>[2x]MAATVWQPLNPGAGGQVQDVVADPNQANVVYMASDMEGVYKSTNNGESWQITGNLVNNRVFAVA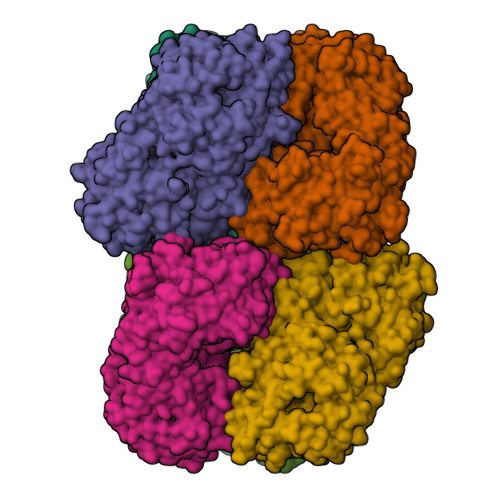VTPGNSNKIFVGTLYGLHISTNGSNSYALVPETENKSIASIAFKPGNANHIIAAPGWRDDDDFIGKFGETAAGPGQVFVSQNGGSSWQTVTFDSNSSTDRNVYSVVFDQSNANTVYLGSNKGVYKSTNGGLNWQRIAGPDDAVRPWNKGIALSPNGQVLYATYAEAKPDLRYNTNFLVYATRTSNINWQQVTGGLEGNRRYWYPEVDPRSTGNSHKVLLGAVKDRFGLYEGTFNWDNNGNLTNFYWEKIWDSYDGSWDIGWDYATPPNARFAHYTPVTGGWARGVWSTTNQTMYYASHNSGNNSYSWQNKYSTPTSQTVNWYGTEWPTYKGKGTESTYTYDVAVHENYVIQGQADNGLMESWDGGVSWSNMQHRRGGGFNLSDVQAVDIADAWGVPTVVAQATSGYGGGAHNGRLWAKRLNTHSPADQWVELAGGPNAKAGLPKGVLRDVAVSPANPAKVFMFSSNYGMYMVEDIGRALDYHDRGETLPVTQIYEGLDNSNDARIARKIAPHPTNEKVVFFSSTGGVQGVWRGEQQNDGSWTFAQVLASSGWDAEVEAWAYNGTVYLMSFAKGGGPGLTDGNNWQILLSTDEGQNWQKIFTPADAMAVRPTSNLVWWNSVGNRFKFTGKGGSAGAGNKIVMSYYDHDYQLGYGVFLGTIQSNGQVNWQDITDDLHFSGMTSSRFIKDAGQMYLYSTTPGAGLWRRSISGMNMDPA> MIDTWLAQWGLRLPSSNDATLRLQPAEGPELVMERLEGGWLFVVELGLVPSGLPLGVILQLLQVNSPFSSLAPVKLAADDAGRLVLWAEARDGVDDVDALNRLHDRLREGHSRLVPLLEPTGELVPA;> GSSLRQEPSGQGLGVALKSTPGILSGKLPESVSDVRFSSPQGQGESRTLTDSAGPRQITLRQFENGVTELQLSRPPLTSLVLSGGGAKGAAYPGAMLALEEKGMLDGIRSMSGSSAGGITAALLASGMSPAAFKTLSDKMDLISLLDSSNKKLKLFQHISSEIGASLKKGLGNKIGGFSELLLNVLPRIDSRAEPLERLLRDETRKAVLGQIATHPEVARQPTVAAIASRLQSGSGVTFGDLDRLSAYIPQIKTLNITGTAMFEGRPQLVVFNASHTPDLEVAQAAHISGSFPGVFQKVSLSDQPYQAGVEWTEFQDGGVMINVPVPEMIDKNFDSGPLRRNDNLILEFEGEAGEVAPDRGTRGGALKGWVVGVPALQAREMLQLEGLEELREQTVVVPLKSERGDFSGMLGGTLNFTMPDEIKAHLQERLQERVGEHLEKRLQASERHTFASLDEALLALDDSMLTSVAQQNPEITDGAVAFRQKARDAFTELTVAIVSANGLAGRLKLDEAMRSALQRLDALADTPERLAWLAAELNHADNVDHQQLLDAMRGQTVQSPVLAAALAEAQRRKVAVIAENIRKEVIFPSLYRPGQPDSNVALLRRAEEQLRHATSPAEINQALNDIVDNYSARGFLRFGKPLSSTTVEMAKAWRNKEFT

ExoU is a 687-residue protein that, once translocated through the T3SS, induces cytotoxic effects leading to rapid necrotic cell death; exoU knockout P. aeruginosa strains display greatly decreased virulence in mouse models of acute infection. Notably, ExoU has been shown to carry phospholipase activity with broad substrate specificity which relies on an essential catalytic dyad (Ser142/Asp344), as is the case for other phospholipases. ExoU is expressed by approximately 30% of clinical strains, 90% of which cause acute illness. It is encoded on a pathogenicity island together with its cognate chaperone SpcU, which is required for ExoU's efficient secretion from the bacterial cytoplasm. ExoU forms a 1∶1 complex with SpcU, and folds into three distinct domains, which fulfill catalytic, bridging, and membrane-binding functions.

The structure of the ExoU(30–687)∶SpcU(1–127) complex was solved to a resolution of 2.94 Å by performing a SAD experiment on the selenium edge at the ESRF synchrotron in Grenoble, and harbors a 1∶1 complex in the asymmetric unit. SpcU is a typical type IA chaperone, being composed of a curved, 5-stranded sheet flanked by α-helices. One involves the extremity of the 5-stranded β-sheet, which binds a short β-strand located at the N-terminus of ExoU (residues 62–64), thus generating a 6-stranded sheet. Residues 106–471 delimit the catalytic, phospholipase domain, which is composed of an α/β hydrolase fold with a 6-stranded central β-sheet surrounded by 10 α-helices. The catalytic serine (Ser142) is located at an elbow between β6 and the following helix, in a funnel-like region surrounded by a number of flexible loops. A triple glycine sequence (Gly111, 112, 113), in close proximity, provides its backbone atoms as an oxyanion hole that potentially stabilizes the charge of the transition state intermediate in the phospholipase reaction. In the structure of ExoU, this region is also found to be flexible, and the catalytic aspartate (Asp344) is not traceable in the electron density map, suggesting not only that ExoU could also harbor a ‘cap’ region, but that the structure presented here is in the ‘open ’, and potentially inactive, conformation. Our structure reveals that the C-terminus of ExoU forms a distinct domain (encompassing residues 588–687) that folds into a 4-helical bundle. Interestingly, residues 679, 682, and 683 form a polar, mostly basic ‘backbone’ that could bind to negatively charged eukaryotic phospholipids, and facilitate lipid bilayer recognition. In summary, the structure of ExoU presented here reveals the toxin in its chaperone-bound, inactive, pre-secretion conformation.> MAVPATIPLTITNNSGRAEQIHIYNLGTELSSGRQGWADASGAFHPWPAGGNPPTPAPDASIPGPAPGRSTTIQI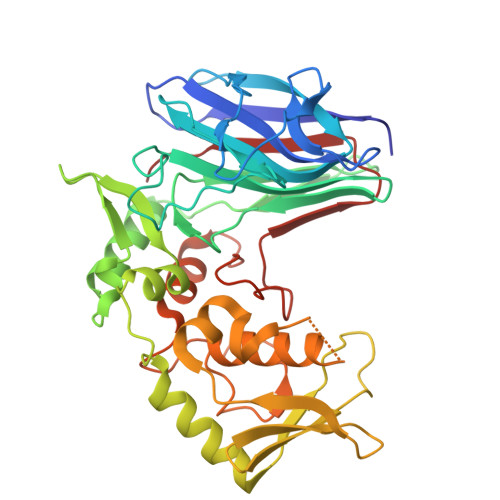PKFSGRIYFSYGRKMEFRLTTGGLVQPAVQNPTDPNRDILFNWSEYTLNDSGLWINSTQVDMFSAPYTVGVRRGDGTTLSTGKLRPGGYNGVFNALRGQSGGWANLIQTRSDGTVLRALSPLYGVETGALPASVMDDYINRVWNKYTGTDLIVTPFADRPDVRYTGRVSGGVLRFTDGSGAVVTTFQKPDASSVFGCHRLLDAPNDQVRGPISRTLCAGFNRTTLLANPHQPDRSAAGFYQEPVTNHYARIIHAHMADGKAYGFAFDDVGHHESLVHDGDPRGASLTLDPFD> GPRRPSVVYLHNAECTGCSESVLRAFEPYIDTLILDTLSLDYHETIMAAAGDAAEAALEQAVNSPHGFIAVVEGGIPTAANGIYGKVANHTMLDICSRILPKAQAVIAYGTCATFGGVQAAKPNPTGAKGVNDALKHLGVKAINIAGCPPNPYNLVGTIVYYLKNKAAPELDSLNRPTMFFGQTVHEQCPRLPHFDAGEFAPSFESEEARKGWCLYELGCKGPVTMNNCPKIK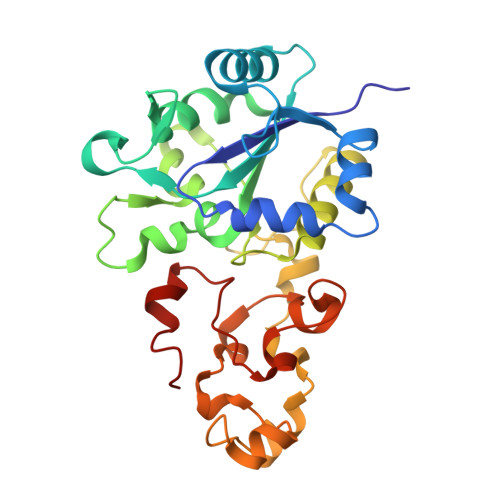FNQTNWPVDAGHPCIGCSEPDFWDAMTPFYQN> EVRNPCACFRNYVPVCGSDGKTYGNPCML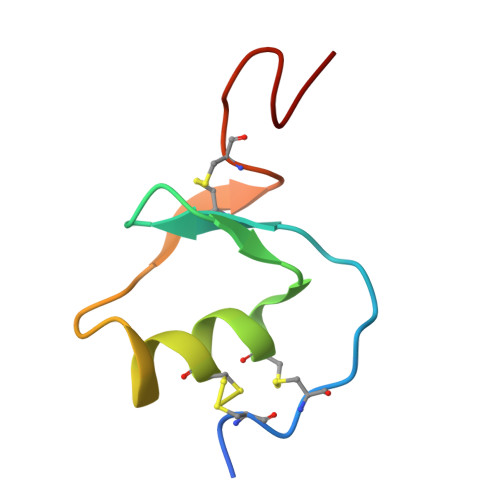NCAAQTKVPGLKLVHEGRCQRSNVEQF> MSAKAISEQTGKELLYKFICTTSAIQNRFKYARVTPDTDWARLLQDHPWLLSQNLVVKPDQLIKRRGKLGLVGVNLTLDGVKSWLKPRLGQEATVGKATGFLKNFLIEPFVPHSQAEEFYVCIYATREGDYVLFHHEGGVDVGDVDAKAQKLLVGVDEKLNPEDIKKHLLVHAPEDKKEILASFISGLFNFYEDLYFTYLEINPLVVTKDGVYVLDLAAKVDATADYICKVKWGDIEFPPPFGREAYPEEAYIADLDAKSGASLKLTLLNPKGRIWTMVAGGGASVVYSDT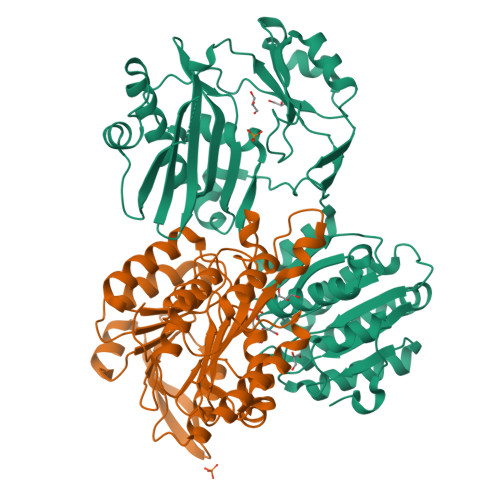ICDLGGVNELANYGEYSGAPSEQQTYDYAKTILSLMTREKHPDGKILIIGGSIANFTNVAATFKGIVRAIRDYQGPLKEHEVTIFVRRGGPNYQEGLRVMGEVGKTTGIPIHVFGTETHMTAIVGMALGHRPIPENLYFQ;> SKSTTLFSRHTKAIVWGMQTRAVQGMLDFDYVCSRDEPSVAAMVYPFTGDHKQKFYWGHKEILIPVFKNMADAMRKHPEVDVLINFASLRSAYDSTMETMNYAQIRTIAIIAEGIPEALTRKLIKKADQKGVTIIGPATVGGIKPGCFKIGNTGGMLDNILASKLYRPGSVAYVSRSGGMSNELNNIISRTTDGVYEGVAIGGDRYPGSTFMDHVLRYQDTPGVKMIVVLGEIGGTEEYKICRGIKEGRLTKPIVCWCIGTCATMFSSEVQFGHAGACANQASETAVAKNQALKEAGVFVPRSFDELGEIIQSVYEDLVANGVI LOBELINE | C22 H27 N O2 | 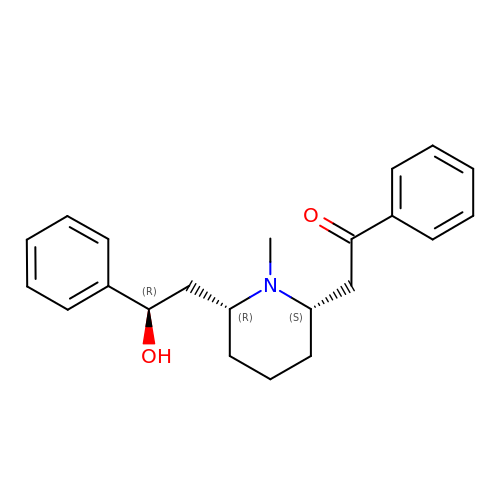MXYUKLILVYORSK-QHAWAJNXSA-N> QVEAIKRGTVIDHIPAQIGFKLLSLFKLTETDQRITIGLNLPSGEMGRKDLIKIENTFLSEDQVDQLALYAPQATVNRIDNYEV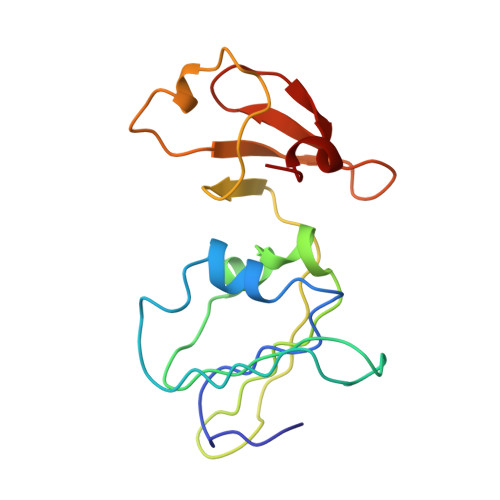VGKSRPSLPERIDNVLVCPNSNCISHAEPVSSSFAVRKRANDIALKCKYCEKEFSHNVVLAN>[2x]GAMGSRKSKAELQSEERKRI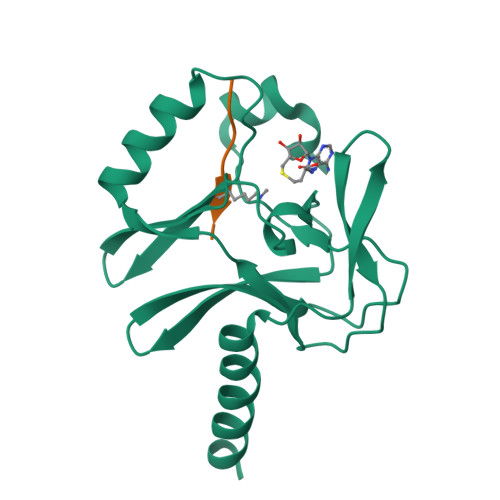DELIESGKEEGMKIDLIDGKGRGVIATKQFSRGDFVVEYHGDLIEITDAKKREALYAQDPSTGCYMYYFQYLSKTYCVDATRETNRLGRLINHSKCGNCQTKLHDIDGVPHLILIASRDIAAGEELLFDYGDRSKASIEAHPWLKH;>AKRHRKVLRD[2x]>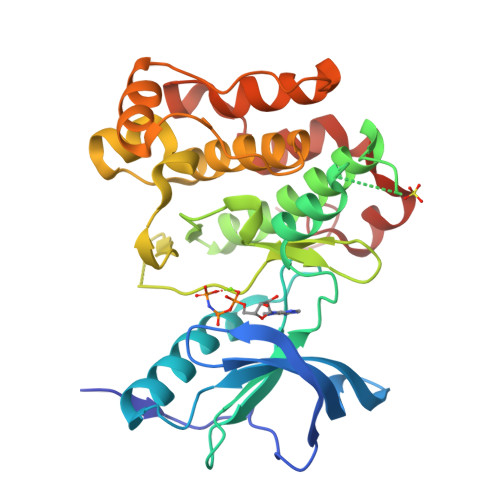GSFSAADVYVPDEWEVAREKITMSRELGQGSFGMVYEGVAKGVVKDEPETRVAIKTVNEAASMRERIEFLNEASVMKEFNCHHVVRLLGVVSQGQPTLVIMELMTRGDLKSYLRSLRPEMENNPVLAPPSLSKMIQMAGEIADGMAYLNANKFVHRDLAARNCMVAEDFTVKIGDFGMTRDIYETDYYRKGGKGLLPVRWMSPESLKDGVFTTYSDVWSFGVVLWEIATLAEQPYQGLSNEQVLRFVMEGGLLDKPDNCPDMLFELMRMCWQYNPKMRPSFLEIISSIKEEMEPGFREVSFYYSEENK[3x]> MSKTVHYLKDYQTPAYHILKTDLHFDINEPQTVVKSRLTVEPQRVGEPLVLDGSAKLLSVKINGAAADYVLEGETLTIAGVPSERFTVEVETEILPAENKSLMGLYASGGNLFTQCEPEGFRKITFYIDRPDVMSKFTTTIVADKKRYPVLLSNGNKIDGGEFSDGRHWVKWEDPFSKPSYLFALVAGDLAVTEDYFTTMSGRNVKIEFYTTEADKPKVGFAVESLKNAMKWDETRFGLEYDLDIFMVVAVGDFNMGAMENKGLNIFNTKFVLADSRTATDTDFEGIESVVGHEYFHNWTGNRVTCRDWFQLSLKEGLTVFRDQEFSGDRASRAVRRIENIRLLRQHQFPEDAGPTAHPVRPASYEEMNNFYTMTVYEKGAEVVRMYHTLLGEEGFQKGMKLYFQRHDGQAVTCDDFRAAMADANGINLDQFALWYSQAGTPVLEAEGRLKNNIFELTVKQTVPPTPDMTDKQPMMIPVKVGLLNRNGEAVAFDYQGKRATEAVLLLTEAEQTFLLEGVTEAVVPSLLRGFSAPVHLNYPYSDDDLLLLLAHDSDAFTRWEAAQTLYRRAVAANLATLSDGVELPKHEKLLAAVEKVISDDLLDNAFKALLLGVPSEAELWDGAENIDPLRYHQAREALLDTLAVHFLPKWHELNRQAAKQENQSYEYSPEAAGWRTLRNVCRAFVLRADPAHIETVAEKYGEMAQNMTHEWGILSA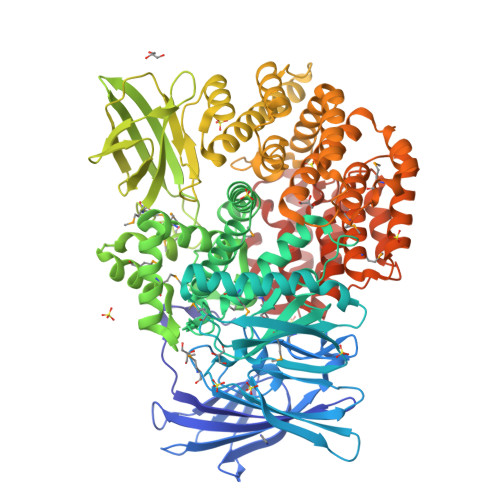VNGNESDTRNRLLAQFADKFSDDALVMDKYFALVGSSRRSDTLQQVRTALQHPKFSLENPNKARSLIGSFSRNVPHFHAEDGSGYRFIADKVIEIDRFNPQVAARLVQAFNLCNKLEPHRKNLVKQALQRIRAQEGLSKDVGEIVGKILD>[6x]MRSIITQICNGVLHGQSYQSGSNDLDKGNSEIFASSLFVHLNEQGKEIIKHKDSDDKI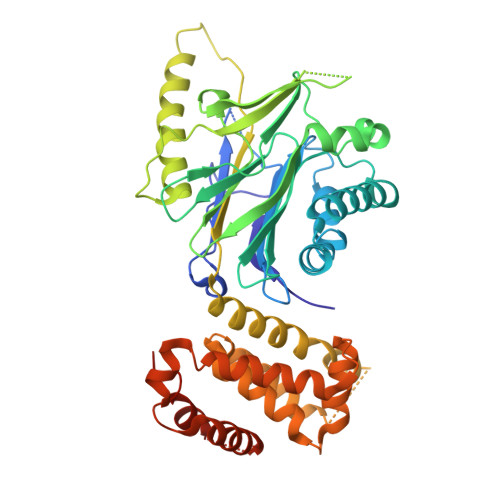VIGYTKDGMAFQIVVDGFYGCERQAVFSFIDNYVLPLIDNFSLDLTRYPDSKKVTESLIHTIYSLRSKHAPLAEFTMSLCVTYQKDEQLFCAGFGIGDTGIAIKRNEGTIEQLVCHTEVDGFKDAFDNYSSANIDLVIERNSVFNTKVMPGDELVGYTYVPPMLEMTEKEFEVETVDGKKINKRIVRHLNLDPGNFDDKDPLFSQLLQVVKSKQKQLVEQAKETGQIQRFGDDFTVGRLVIPDQLLINQLRIHALSIGVSDGLLSYIKNENENKGFLGIYGFFTGADKNIEKATLYKNLIAKYQNNHFISLIILSALVSDSKTPLMTQYLVGYLDFPSKALLANKITELLLKELENPDMREILGSRLATDVIEELETKIIRYIHNPAGSDIHSTLNLWTADKIKAATNSSLTI>[2x]MHRTSNGSHATGGNLPDVASHYPVAYEQTLDGTVGFVIDEMTPERATASVEVTDTLRQRWGLVHGGAYCALAAMLATEATVAVVHEKGMMAVGQSNHTSFFRPVKEGHVRAE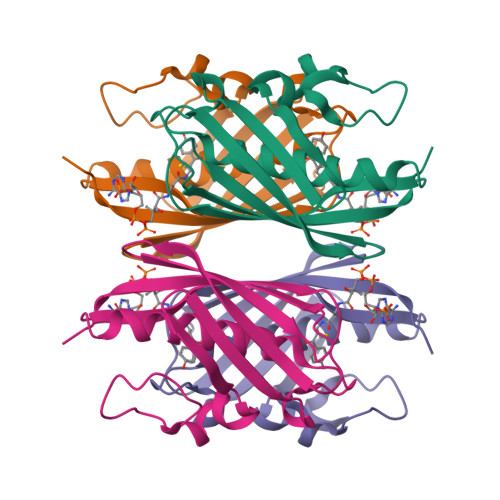AVRIHAGSTTWFWDVSLRDDAGRLCAVSSMSIAVRPRRD>AEASVDIQGNDQMQFNTNAITVDKSAKQFTVNLSHPGNLPKNVMGHNWVLSTAADMQGVVTDGMASGLDKDYLKPDDSRVIAHTKLIGSGEKDSVTFDVSKL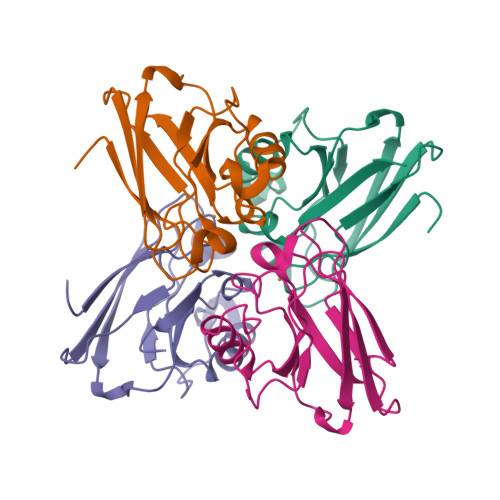KEGEQYMFFCTFPGHSALMKGTLTLK[4x]Viruses acquire host genes via horizontal gene transfer and can express them to manipulate host biology during infections. Some viral and host homologs retain sequence identity, but evolutionary divergence can obscure host origins. We used structural modeling to compare vaccinia virus proteins with metazoan proteomes. We identified vaccinia A47L as a homolog of gasdermins, the executioners of pyroptosis.

An X-ray crystal structure of A47 confirmed this homology and cell-based assays revealed that A47 inhibits pyroptosis. Our findings demonstrate the potential of structural homology screens to reveal genes that viruses capture from hosts and repurpose to benefit viral fitness.

> SNNAVTHVSANSIRQHILFNNFETLHKDIQSKIDLVNTFTPQTKNLIFRNLLIVITNSYHLQNLLDALEQLEPMYVTDAYSEAILNEIGLCDKGIPNLSSIHFMIYLVSGLTKLTTKQSKILMEIVTDAKIFCHHVNVLEYIIKKNVEKLETVTSTLLEKYTKLPLEVTLFKESGLKIQGNTYIWDPEHKKSICNLYTVIKIMSYIM> SFTMAQQSGGGLTRGSFPEGFVFGTASAAYQYEGAVKEDGRGQTIWDTFAHTFGKITDFSNADVAVDQYHRFEEDIQLMADMGMDAYRFSI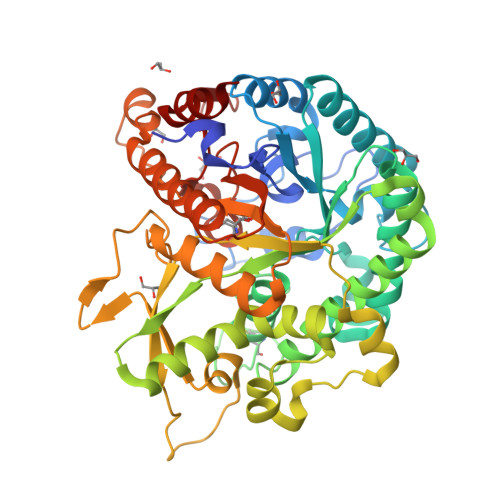AWSRIYPNGVGQVNQAGIDHYNKLIDALLAKGIQPYVTLYHWDLPQALEDKYKGWLDRQIVDDFAAYAETCFREFGDRVKHWITLNEPHTVAIQGYDAGLQAPGRCSVLLHLYCKAGNSGTEPYVVAHHFILAHAAAASIYRTKYKATQNGQLGIAFDVMWFEPMSNTTIDIEAAKRAQEFQLGWFADPFFFGDYPATMRARVGERLPRFTADEAAVVKGALDFVGINHYTTYYTRHNNTNIIGTLLNNTLADTGTVSLPFKNGKPIGDRANSIWLYIVPRGMRSLMNYVKERYNSPPVYITENGMDDSNNPFISIKDALKDSKRIKYHNDYLTNLAASIKEDGCDVRGYFAWSLLDNWEWAAGYSSRFGLYFVDYKDNLKRYPKNSVQWFKALLKT> MYALAIALLAFSTFVSNAFANKEYLLLDIRDATTSEIISALRDVEIELKVKAKGIARHLIVVKQNDANLQKLGEIDIPGRSCSTPVEDLDNLMEDIGISWPRNELTNVNVTLFERTLDLKDKTMEQFWSEAKAYGQLVKPVLSSFTYRAFKANGAYPPKVYFFVNLPRENLN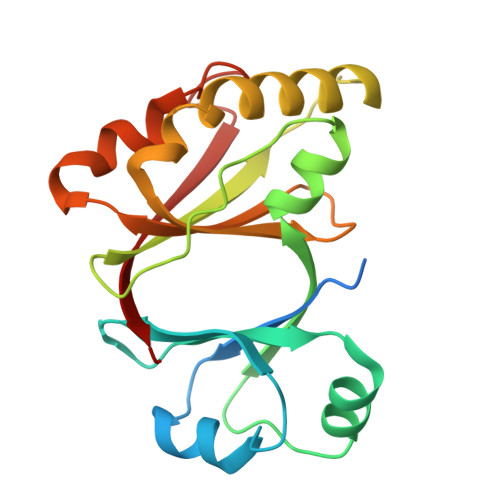DASSKGIDIFGGPGKARTTVQYVTKLS>[2x]SN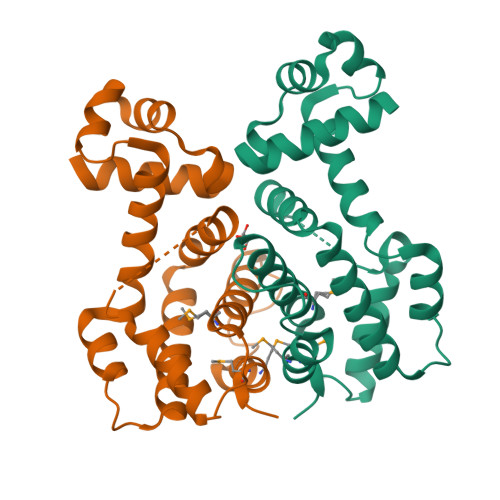AMKKKDMNKQVKIQDAVAAIILAEGPAGVSTTKVAKRVGIAQSNVYLYFKNKQALIDSVYARETNRILSTTDLDRLSDSTIDVTTRIRLYVQQVYDYSLANPDSLTIIQQIKALNGQGMTISAADADPNNIVANLLTAAIDAKVIKQLPVSLHMGVVFSTIHTHTTNISKGRYAQDQYTFGDIFQMIWDAMKQD>[2x]TTHTSDFLKLNPSSGLWPASGLGQDVIVAVLDSGIWPESASFQDDGMPEIPKRWKGICKPGTQFNASMCNRKLIGANYFNKGILANDPTVNITMNSARDTDGHGTHCASITAGNFAKGVSHFGYAPGTARGVAPRARLAVYKFSFNEGTFTSDLIAAMDQAVADGVDMISISYGYRFIPLYEDAISIASFGAMMKGVLVSASAGNRGPGIGSLNNGSPWILCVASGHTDRTFAGTLTLGNGLKIRGWSLFPARAFVRDSPVIYNKTLSDCSSEELLSQVENPENTIVICDDNGDFSDQMRIITRARLKAAIFISEDPGVFRSATFPNPGVVVNKKEGKQVINYVKNSVTPTATITFQETYLDTKPAPVVAASSARGPSRSYLGISKPDILAPGVLILAAYPPNVFATSIGTNILLSTDYILESGTSMAAPHAAGIAAMLKAAHPEWSPSAIRSAMMTTADPLDNTRKPIKDSDNNKAATPLDMGAGHVDPNRALDPGLVY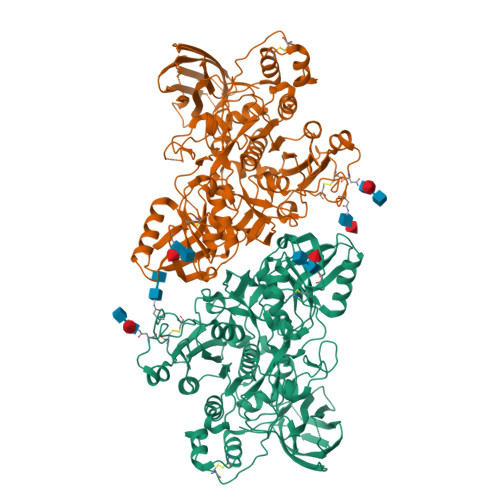DATPQDYVNLLCSLNFTEEQFKTIARSSASHNCSNPSADLNYPSFIALYSIEGNFTLLEQKFKRTVTNVGKGAATYKAKLKAPKNSTISVSPQILVFKNKNEKQSYTLTIRYIGDEGQSRNVGSITWVEQNGNHSVRSPIVTSPIIEVW> UGCGUCACACCGGUGAAGUCGC;> GCGUCAC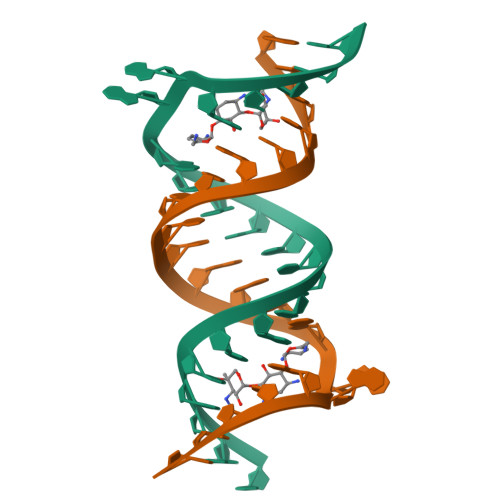ACCGGUGAAGUCGC>MERKQSNAHSTFADINEVEDEAEQELQQQENNNNKRFSGNRGPNRGKQRPFRGFSRQVSLETGFSVLNRESRERDDKKSLPRSGRSFGGFESGGIINGGDGRKTDFSMFRTKSTLSKQKSLLPSIIRERDIENSLRTEDGETKDDSINENVSAGRYFAALRGPELDEVKDNEDILLPKEEQWPFLLRFPIGCFGICLGLSSQAVLWLALAKSPATNFLHITPLINLVVWLFSLVVLVSVSFTYILKCIFYFEAVKREYFHPVRVNFFFAPWVVCMFLAISVPPMFSPNRKYLHPAIWCVFMGPYFFLELKIYGQWLSGGKRRLCKVANPSSHLSVVGNFVGAILASKVGWDEVAKFLWAVGFAHYLVVFVTLYQRLPTSEALPKELHPVYSMFIAAPSAASIAWNTIYGQFDGCSRTCFFIALFLYISLVARINFFTGFKFSVAWWSYTFPMTTASVATIKYAEAVPGYPSRALALTLSFISTAMVCVLFVSTLLHAFVWQTLFPNDLAIAITKRKLTREKKPFK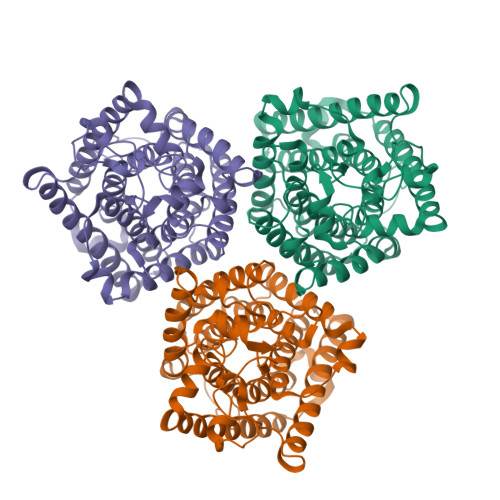RAYDLKRWTKQALAKKISAEKDFEAEEESHH[3x]>[2x]SPRANEIKKGMVLNYNGKLLLVKDIDIQSPTARGAATLYKMRFSDVRTGLKVEERFKGDDIVDTVTLTRRYVDFSYVDGNEYVFMDKEDYTPYTFTKDQIEEELLFMPEGGMPDMQVLTWDGQLLALELPQTVDLEIVETAPGIKGASASARNKPATLSTGLVIQVPEYLSPGEKIRIHIEERRYMGRAD

In bacteria, EF-P plays an important role in overcoming such polyproline sequence-induced ribosome stalling. Additionally, numerous bacteria possess an EF-P paralog called EfpL (also known as YeiP) of unknown function. Here, we functionally and structurally characterize EfpL from Escherichia coli and demonstrate its role in the translational stress response. Bioinformatic analyses based on AlphaFold predictions indicate that EF-P-like proteins have a three-domain structure similar to EF-P, but they only share about 30% sequence similarity.

In the frame of this study, we solve the structure of E. coli EfpL (EfpL) and uncover its role in translation of XP(P)X-containing proteins: Through ribosome profiling, we explore the EfpL arrest motif spectrum and uncover additional sequences beyond the typical polyproline motifs that both EF-P and EfpL can resolve. The EfpL structure reveals a significantly tilted KOW domain relative to the C-terminal di-domain compared to EF-P structures, certainly enabled by the flexible hinge region between the independent moieties. However, a separate alignment of KOW and OB di-domains between E. coli EfpL and for example, the EF-P structure resolved within the E. coli ribosome from Huter et al., reveals low r.m.s.d. values. This suggests the relative domain arrangement is merely a consequence of the unique crystal packing. The structural alignment ultimately revealed a β3Ωβ4 loop elongation by two amino acids for EfpL, different from the canonical seven amino acids in EF-P. In this way, EfpL_R33 remains apical similar to canonical EF-Ps. As shown by the lowest-energy model, the local geometry in principle would allow the unmodified arginine of the EfpL β3Ωβ4 loop to reestablish the interaction with the tRNA trinucleotide. Furthermore, the model suggests EfpL could mediate specific interactions with the RNA as—unlike EF-P_K34—EfpL_R33 was found to stack between the two C-bases and make polar interactions with the phosphate-sugar backbone. Hence, based on the docking model we suggest that the prolonged β3Ωβ4 loop and its central tip R33 are capable of compensating for the lack of a modified lysine. A literature search revealed that E. coli EfpL is acylated at four different lysines (K23, K40, K51, and K57) in the KOW domain.4-(piperidin-1-yl)-1,2,5-oxadiazol-3-amine 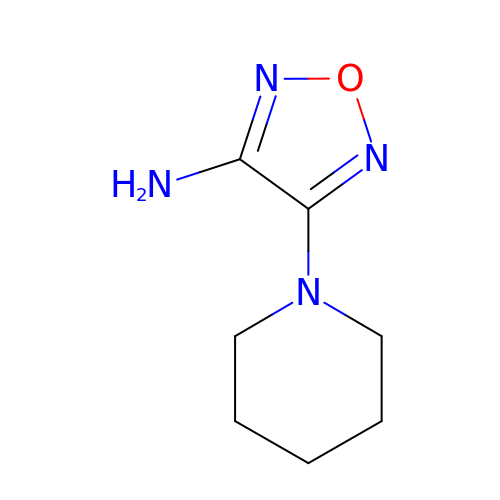| C7 H12 N4 O | RVSIGDHRHURXCQ-UHFFFAOYSA-N>MGSSHHHHHHGENLYFQSTKKSAAEASKKPRQKRTATKAYNVTQAFGRRGPE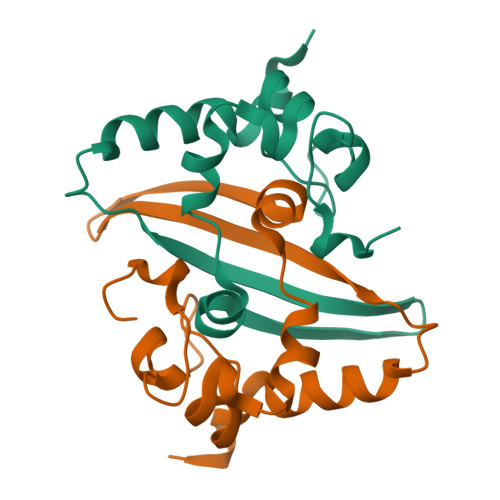QTQGNFGDQELIRQGTDYKHWPQIAQFAPSASAFFGMSRIGMEVTPSGTWLTYTGAIKLDDKDPNFKDQVILLNKHIDAYKTFP[4x]> DEAGITGTWYNQLGSTFIVTAGADGALTGTYESAVGNAESRYVLTGRYDSAPATDG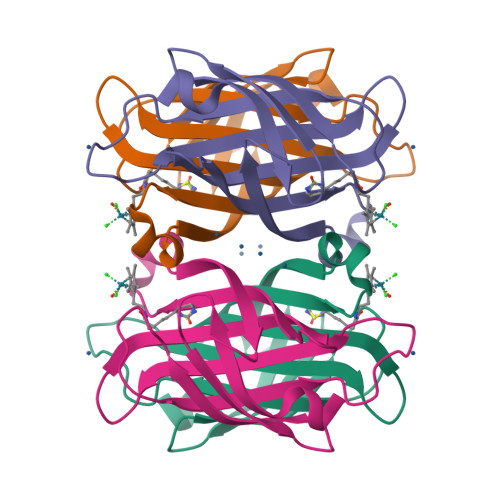SGTALGWTVAWKNNYRNAHSATTWSGQYVGGAEARINTQWLLTYGTTEANAWESTLVGHDTFTKVK> GAAAEPILEVLVGKVLEQGLMEVLEEEELAAMRAHQEHFEQIRNAELVATQRMEAAERRKLEEKERRMQQERERVERERVVRQKVAASAFARGYLSGIVNTVFDRLVSSGYIYDPVMREVETAFMPWLKEQAIGYLARGVVARRVVDKLVEDAAAALAANRSTLADKAASTAATVDAWAERQAKMEAELQGKELEAVRRRPTFVLRELKPAVASADAVEAAAAELTAQ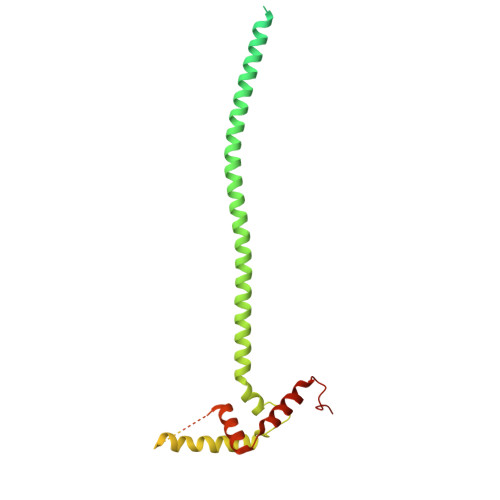AEEAANAKWEADKAEAAEKARAEAEAAAEEQKALLEELAATAAAEAEERGEEPPAEPPSLPDGVEPVDVEAEVAKAVEAVPKPPVKEVTDIDILSYMMDKGAITKDAIIQALAVHALGDKAYTNHPAFAEAEGA> MEQAMRERSELARKGIARAKSVVALAYAGGVLFVAENPSRSLQKISELYDRVGFAAAGKFNEFDNLRRGGIQFADTRGYAYDRRDVTGRQLANVYAQTLGTIFTEQAKPYEVELCVAEVAHYGETKRPELYRITYDGSIADE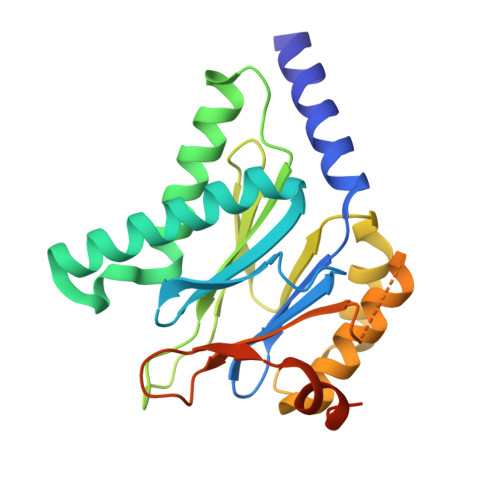PHFVVMGGTTEPIANALKESYAENASLTDALRIAVAALRAGSADTSGGDQPTLGVASLEVAVLDANRPRRAFRRITGSALQALLVDQESPQSDGESSG>[7x]AKDVKFGADARALMLQGVDLLADAVAVTMGPKGRTVIIEQSWGSPK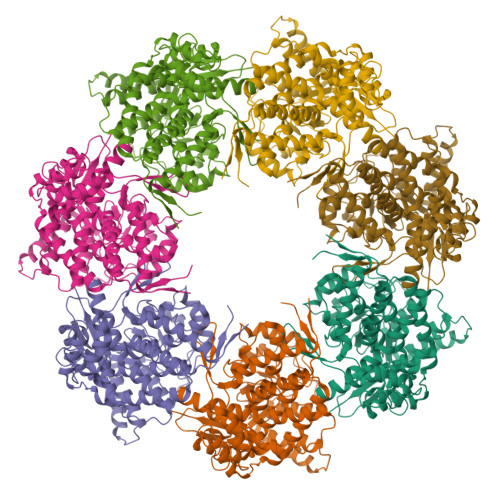VTKDGVTVAKSIDLKDKYKNIGAKLVQDVANNTNEEAGDGTTTATVLARSIAKEGFEKISKGANPVEIRRGVMLAVDAVIAELKKQSKPVTTPEEIAQVATISANGDKEIGNIISDAMKKVGRKGVITVKDGKTLNDELEIIEGMKFDRGYISPYFINTSKGQKCEFQDAYVLLSEKKISSIQSIVPALEIANAHRKPLVIIAEDVDGEALSTLVLNRLKVGLQVVAVKAPGFGDNRKNQLKDMAIATGGAVFGEEGLTLNLEDVQPHDLGKVGEVIVTKDDAMLLKGKGDKAQIEKRIQEIIEQLDVTTSEYEKEKLNERLAKLSDGVAVLKVGGTSDVEVNEKKDRVTDALNATRAAVEEGIVLGGGCALLRCIPALDSLTPANEDQKIGIEIIKRTLKIPAMTIAKNAGVEGSLIVEKIMQSSSEVGYDAMAGDFVNMVEKGIIDPTKVVRTALLDAAGVASLLTTAEVVVTEIP2-(2-methyl-1,3-thiazol-4-yl)-1-(morpholin-4-yl)ethan-1-one | C10 H14 N2 O2 S | 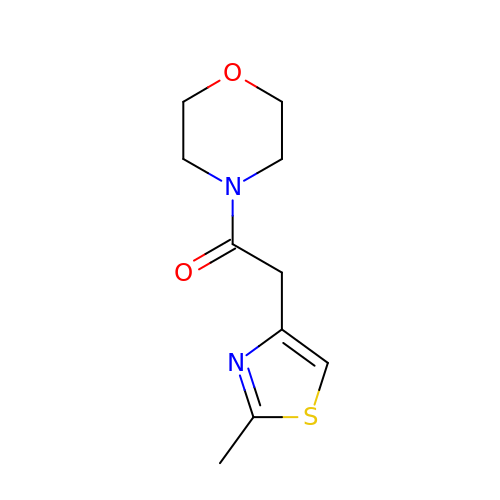ZGUYZZRXRYNXNN-UHFFFAOYSA-N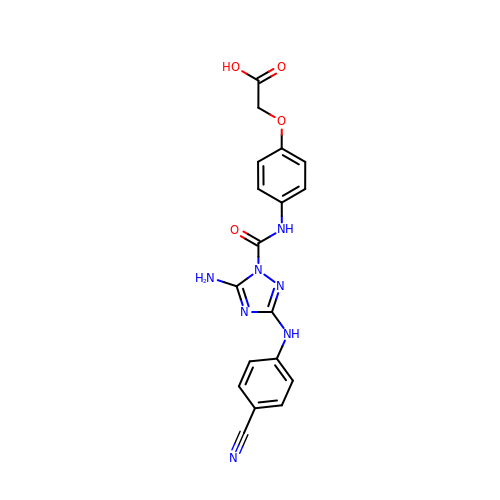[4-({5-amino-3-[(4-cyanophenyl)amino]-1H-1,2,4-triazole-1-carbonyl}amino)phenoxy]acetic acid | C18 H15 N7 O4 | TWAPQXNNCFSTFQ-UHFFFAOYSA-N methoxy-[(~{E},3~{R})-3-[(2~{R})-1-methoxy-1,3-bis(oxidanylidene)butan-2-yl]tridec-11-enyl]phosphinous acid | C19 H35 O6 P | 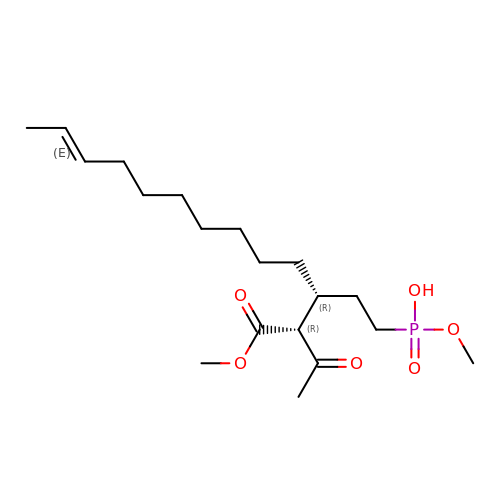KFPPYXMTKZSOKI-VGRIIWOTSA-N>ANNHIRTVLKLFRTIDLDDSKKSFYLTAAKYGIQTQLREPIIRIVGGYLPSTKLSEACVKNMISEVYEIEGDF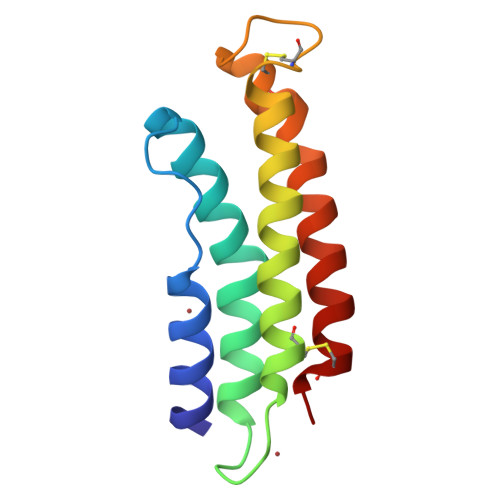YSKFSYACEDHAPYSVECLEDARDDYLTQLVELFKETKKCLRE[3x]>MSEVEFSHEYWMRHALTLAKRARDERGVPVGAVLVLNNRVIGEGWNRANGLHDPTAHAEIMALRQGGLVMQNYRLYDATLYSTFEPCVMCAGAMIHSRIGRVVFGVRNAKTGAAGSLMDVLHHPGMNHRVEIT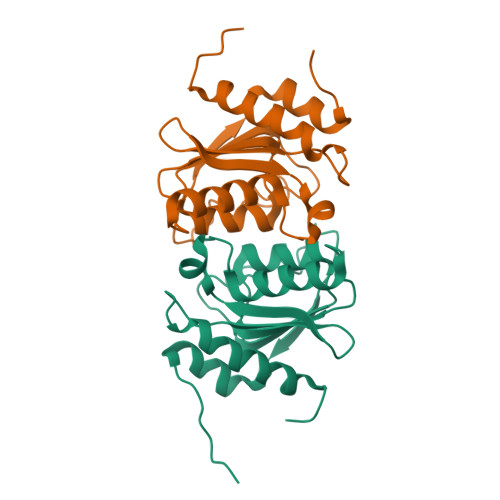EGILADECAALLCRFFRMPRRVFNAQKKAQSSTD[8x]> MTQAEIKLCSLLLQEHFGEIVEKIGVHLIRTGSQPLRVIAHDTGTSLDQVKKALCVLVQHNLVSYQVHKRGVVEYEAQCSRVLRMLRYPRYIYTTKTLYSDTGELIVEELLLNGKLTMSAVVKKVADRLTETMEDGKTMDYAEVSNTFVRLADTHFVQRCPSVPTTENSDPGPPPPAPTLVINEKDMYLVPKLSLIGKGKRRRSSDEDAAGEPKAKRPKYTTDNKEPIPDDGIYWQANLDRFHQHFRDQAIVSAVANRMDQTSSEIVRTMLRMSEITTSSSAPFTQPLSSNEIFRSLPVGYNISKQVLDQYLTLLADDPLEFVGKSGDSGGGMYVINLHKALASLATATLESVVQERFGSRCARIFRLVLQKKHIEQKQVEDFAMIPAKEAKDMLYKMLSENFMSLQEIPKTPDHAPSRTFYLYTVNILSAARMLLHRCYKSIANLIERRQFETKENKRLLEKSQRVEAIIASMQATGAEEAQLQEIE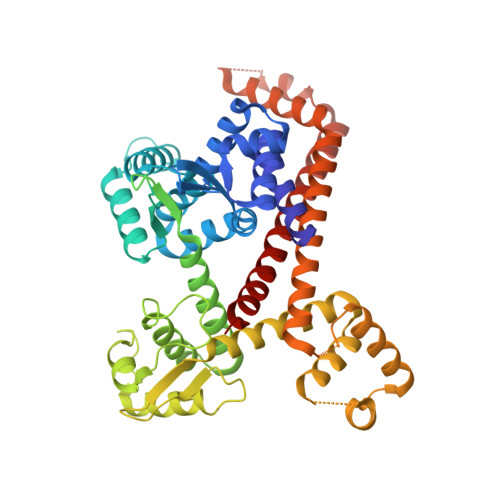EMITAPERQQLETLKRNVNKLDASEIQVDETIFLLESYIECTMKRQ>[2x]SNAMGEV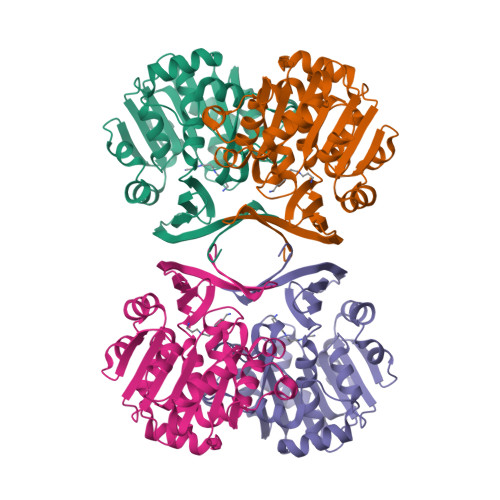AYTNGNGNDKSHSPPNGYRKSCWYEEEIEENLRWCFALNSILHTGASQYQDIALLDTKPFGKALVLDGKLQSAETDEFIYHECLVHPALLHHPMPKNVFIMGGGEGSTARELLRHKTIDKVVMCDIDEEVVEFCKSYLVVNKEAFHDSRLEVVINDAKAELEGKEEKYDVIVGDLADPIEGGPCYKLYTKDFYELTLKPKLKKGGIFVTQAGPAGIFSHTEVFSCIYNTLRQVFKYVVPYSAHIPSYADIWGWVLASDSPLDLSAEELDIRMRQRIIEENRYLDGKTFVSSSTLSKAVRNSLNNETHVYTEGAARFIYGHGKNA Further, the in vitro assay confirmed that NasF5053 could produce NAS-C (47.4%), Asp-A (44.4%), as well as a minor product NAS-B (8.2%) (trace I). NasF5053 adopts the prism-like fold characteristic for P450s, consisting of a large domain of 10-helices (C-L) and a small domain of four α-helices (A, B, B’, and K’) and three β-sheets (strands β1-1 to 4, β2-1 to 2, and β3-1 to 2). Our systematic mutagenesis studies on the promiscuous NasF5053 and the versatile NascB identified four key resides, Q65, A86, S284, and V288, which play critical roles in controlling product regio-configurations and stereo-configurations. To obtain insights into the structural basis for regio-specificity, stereo-specificity, and chemical versatility, we further determined high-resolution crystal structures of wild-type NasF5053 in its substrate-free and substrate-bound form, and of two NasF5053 mutants (Q65I-A86G and S284A-V288A) in their substrate-bound forms.

On the other hand, the single mutations Q65I and A86G in NasF5053 dramatically reduced the production of NAS-C (trace IV). Furthermore, the double mutation A86G-Q65I almost abolished the production of NAS-C, leaving ASP-A as the only detectable product (trace VI). These results clearly indicate that Q65 and A86 are the two crucial residues in NasF5053 that that direct the enzyme to produce NAS-C. Comparisons among the three substrate-bound structures showed that all substrate-interacting residues, the heme, and the two substrates superimpose well (RMSD in this region between any two structures <0.26 Å), except for the mutated residues and the adjacent residues such as K289 and I87. The plotting of the spectral variation as a function of cWL-PL concentration is fitting to a rectangular hyperbola curve, yielding a binding constant of 11.6 ± 2.1 µM for the interaction between cWL-PL and wild-type NasF5053, 25.6 ± 1.0 µM for cWL-PL with NasF5053-Q65I-A86G and 4.81 ± 0.26 µM for cWL-PL with NasF5053-S284A-V288A. The Q65-A86 patch is involved in regulating the motion of the long loop αB’-αC, where Q65 and A86 reside at its two ends. The Q65I and A86G mutations result in a shift of the αB’-αC loop away from cWL-PL-U radical. The consequent relaxation of the restraints on Int1 unfolds Int1 (the distance between N10 and C2 is approximately 4.7 Å in most distance distributions). The results exclude the intramolecular cyclization of the cWL-PL-U radical to form a pyrroloindoline, without affecting the formation of ASP-A; this observation is consistent with our data that NasF5053-Q65I-A86G exclusively produce Asp-A.

> GSTLTYPFHDWSQELSPRYAQLRASDAPVCPVVSEGTGDPLWLVTRYATAVKLLEDSRFSSEAAIASGAPRQEPVELRAPGTRGDGIAMLREAGLRSVLADGLGPRAVRRHQGWINDLAETLMSELASREGTFDLAADFVEPLSSALVSRTLLGELSADERDLLAHCADTGLRFCGVTHEEQVHAFTQMHEFFLEHARRLAGTPGEHLLKLIAEAPVDQGPLSDEALAEAGSLLVVAGFPTSSGFLCGALLTLLRHPDAVQELHAHPERVPSAVEELLRYTPLSTGSVKRMATEDLEIDGVRIKAGEVVMVSLEAVNHDPDAFEDPDVFRPGREGPMHFGFGRGRHFCPGNRLARCVIEATVRAVARRPGLRLAVAPEEISWHEGLFFRRPRAIPATW>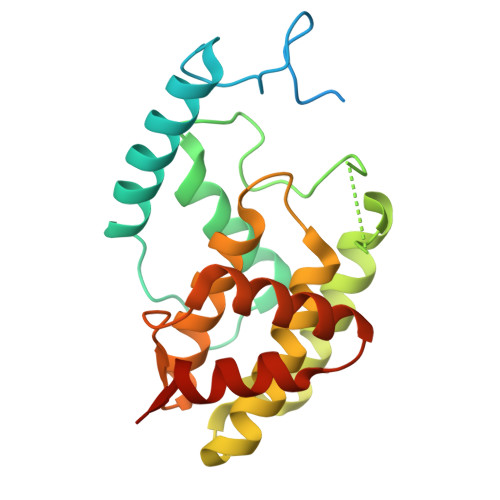 MGSSHHHHHHSQDPNSSSARLQVEMGDKFGEGRDPYLYPGLDIMRNRLNIHQQQRLEQAAYEMTALRAATIELGPLVRGLPHLRTIHRQLYQDIFDWAGQLREVDIYQGDTPFCHFAYIEKEGNALMQDLEEEGYLVGLEKAKFVERLAHYYCEINVLHPFRVGSGLAQRIFFEQLAIHAGYQLSWQGIEKEAWNQANQSGAMGDLTALQMIFSKVVSEAGESE> AAKRRPKEAEPEQVAPETPEDRDEDEREEKRRKTTRKKLESHTVPVQSRSERKAAQSKSVIPKINSPKCPECGQHLDDPNLKYQQHPEDAVDEPQMLTSEKLSIYDSTSTWFDTYEDSPMHRFTSFSVYCSRGHLCPVDTGLIEKNVELYFSGCAKAIHDENPSMEGGINGKNLGPINQWWLSGFDGGEKVLIGFSTAFAEYILMEPSKEYEPIFGLMQEKIYISKIVVEFLQNNPDAVYEDLINKIETTVPPSTINVNRFTEDSLLRHAQFVVSQVESYDEAKDDDETPIFLSPCMRALIHLAGVSLGQRRATRRVMGATKEKDKAPTKATTTKLVYQIFDTFFSEQIEKYDKEDKENAMKRRRCGVCEVCQQPECGKCKACKDMVKFGGTGRSKQACLKRRCPNLAVKEADDDEEADDDVSEMPSPKKLHQGKKKKQNKDRISWLGQPMKIEENRTYYQKVSIDEEMLEVGDCVSVIPDDSSKPLYLARVTALWEDKNGQMMFHAHWFCAGTDTVLGATSDPLELFLVGECENMQLSYIHSKVKVIYKAPSENWAMEGGTDPETTLPGAEDGKTYFFQLWYNQEYARFESPPKTQPTEDNKHKFCLSCIRLAELRQKEMPKVLEQIEEVDGR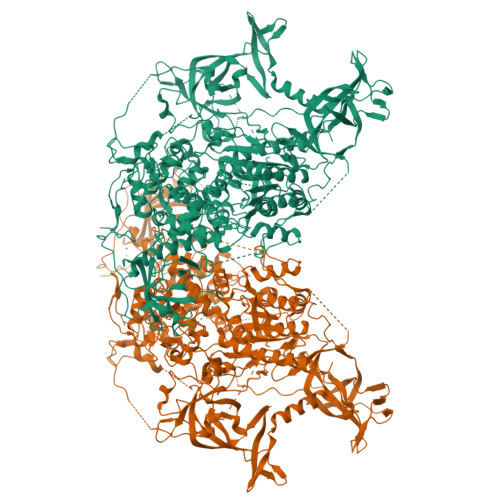VYCSSITKNGVVYRLGDSVYLPPEAFTFNIKVASPVKRPKKDPVNETLYPEHYRKYSDYIKGSNLDAPEPYRIGRIKEIHCGKKKGKVNEADIKLRLYKFYRPENTHRSYNGSYHTDINMLYWSDEEAVVNFSDVQGRCTVEYGEDLLESIQDYSQGGPDRFYFLEAYNSKTKNFEDPPNHARSPGNKGKGKGKGKGKGKHQVSEPKEPEAAIKLPKLRTLDVFSGCGGLSEGFHQAGISETLWAIEMWDPAAQAFRLNNPGTTVFTEDCNVLLKLVMAGEVTNSLGQRLPQKGDVEMLCGGPPCQGFSGMNRFNSRTYSKFKNSLVVSFLSYCDYYRPRFFLLENVRNFVSYRRSMVLKLTLRCLVRMGYQCTFGVLQAGQYGVAQTRRRAIILAAAPGEKLPLFPEPLHVFAPRACQLSVVVDDKKFVSNITRLSSGPFRTITVRDTMSDLPEIQNGASNSEIPYNGEPLSWFQRQLRGSHYQPILRDHICKDMSPLVAARMRHIPLFPGSDWRDLPNIQVRLGDGVIAHKLQYTFHDVKNGYSSTGALRGVCSCAEGKACDPESRQFSTLIPWCLPHAGNRHNHWAGLYGRLEWDGFFSTTVTNPEPMGKQGRVLHPEQHRVVSVRECARSQGFPDSYRFFGNILDRHRQVGNAVPPPLAKAIGLEIKLCLLSSARESASAAVKAKEEAATKD Pygo proteins promote Armadillo- and β-catenin-dependent transcription, by relieving Groucho-dependent repression of Wnt targets. Their PHD fingers bind histone H3 tail methylated at lysine 4, and to the HD1 domain of their Legless/BCL9 cofactors, linking Pygo to Armadillo/β-catenin. Lgs/BCL9 proteins are adaptors between Pygo and Armadillo/β-catenin, binding to Pygo PHD fingers through their homology domain 1 (HD1) and to Armadillo/β-catenin through their homology domain 2 (HD2; Kramps et al., 2002; Städeli and Basler, 2005). Intriguingly, fly Pygo orthologs exhibit a tryptophan > phenylalanine substitution in their histone pocket-divider which reduces their affinity for histones.

To resolve this, and to investigate how the deviant pocket-divider of the Pygo PHD finger affects histone binding, we solved the crystal structure of the Drosophila PHD-HD1 complex and examined its H3K4me binding by nuclear magnetic resonance (NMR) spectroscopy. Although dPHD-HD1 is far less stable than the human complexes, we obtained diffracting crystals under several conditions, which allowed us to solve its structure at 2.7 Å resolution. An important structural consequence of the W > F substitution is a significant widening of the T3 channel: this is bordered on one side by F773 the phenyl ring of which is less protruberant than the indole ring of a typical W pocket-divider. This is partially compensated for by a T > N substitution at the opposite channel wall where the bulky side chain of N790 protrudes into the unliganded channel and thus narrows it. Abutting the F pocket-divider in fly Pygo is a striking groove, walled by F773 and E767, and floored by the aromatic ring of F765. This groove is not seen in human Pygo in which a conserved L (L345) fills out the equivalent space, substituting for F765, as already mentioned. Key for the interaction between PHD and HD1 is a hydrogen bond between an invariant T in HD1 α1 (T328) and W797, the PHD signature residue (Bienz, 2006). The topological equivalent of this allosteric triplet in the fly complex is W797, L781, and V764: W797 and L781 engage in crucial interactions with T328, and also connect with V764, a residue lining the T3 channel.

>[18x]GAMANHIFVFSTQLANKGAESVLSGQFQTIIAYHCTQ;>[15x]GAMAIYPCGMCHKEVNDNDEAVFCESGCNFFFHRTCVGLTEAAFQMLNKEVFAEWCCDKCVS;>[3x]AAMAIYPCGMCHKEVNDNDEAVFCESGCNFFFHRTCVGLTEAAFQMLNKEVFAEWCCDKCVS>[2x]MSDSRLAEAAHSSFARHETFAPRFGWLHKAYMQVQSNPEAFLADDAPVQLG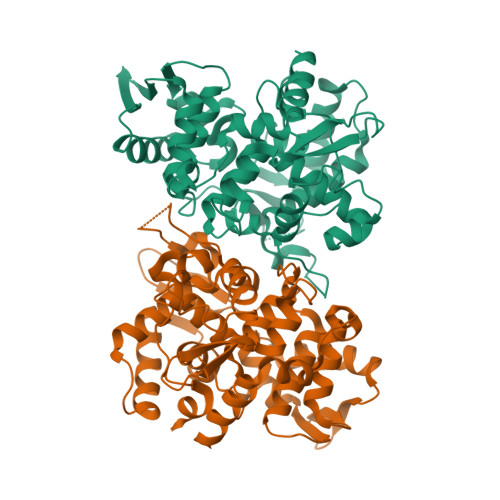VGKNMVYAMRYWSRAFKLTREHYGDDTNSRAMLSYPTWEARWLLDEDGADPYLEELGSLWLLHWWLLSSRPGTKSWAPSWYVAFHLAPFSRFTLADLTQVIVRHVNLSFPEGPVEASIAKDVDCITKMYVPAQRLRGGAPGAFEDLLSCPFRELGLMEQVGQRGSSEWEFTSGSRPSLPARIIAYACLDYAARTTRNAGSISLARLANEPGAPGRAFRIREADIAAALEKVAASHQELQLVEAVGQRSLTFTSGPFDLAWDVLDEQYDNVRSRPNFPTREDWARRYPKLAEAEKRELKQLDIIDPQLALTEETV3-(3-chlorophenyl)-5-methyl-1H-pyrazole | C10 H9 Cl N2 | 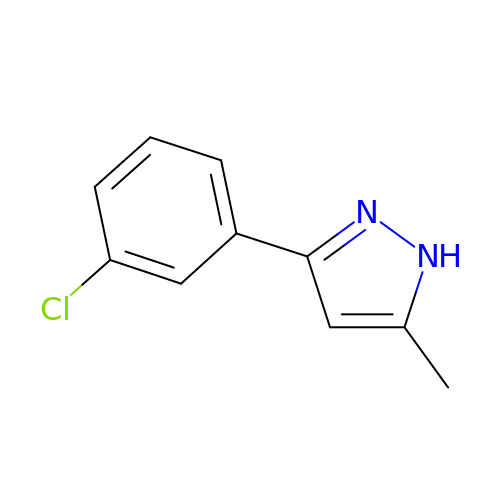KOMMMAVILXYEJR-UHFFFAOYSA-N> LPAVVGLS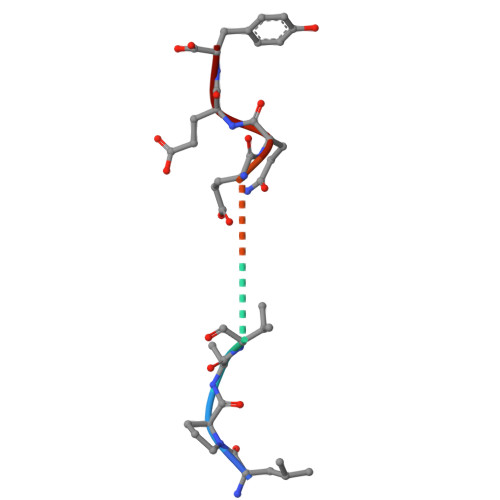PGEQEY> SMGVRKLATIRTAGEITPIAGAEAIECCHVDGWTCVIKKGEFKQGDRGVYFEIDSFIKEDNDRYPMLSKQVIDYEGQRGTRLRTARLRGQLSQGLFLPMDRFPELASNQVGDDVTE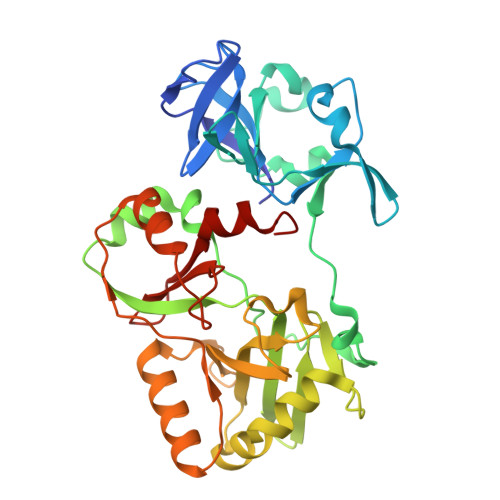ILGITKWEPPISTNLSGEILGEFPTFISKTDQERVQNLIPQIEENKGQKFEVTVALDGSSMTVYRKDDHIGVCGRNWELRETATNAQWHAARRNKMIEGLQFLNRNLALQGEIIGESIQGNLEKLKGQDFYLFDIYDIDKAQYLTPIERQSLVKQLNDNGFTVKHVPILDDLELNHTAEQILAMADGPSLNKNVKREGLVFKRLDGKFSFKAISNAYLEKHKDR> TRDFNGTWEMESNENFEGYMKALDIDFATRKIAVRLTFTLVIDQDGDNFKTKATSTFLNYDVDFTVGVEFDEYTKSLDNRHVKALVTWEGDVLVCVQKGEKENRGWKKWIEGDKLYLELTCGDQVCRQVFKK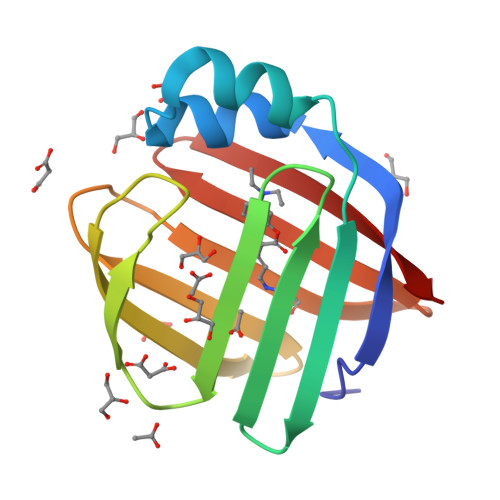K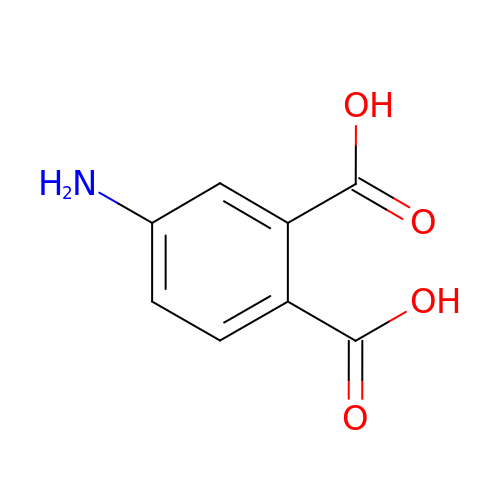4-aminobenzene-1,2-dicarboxylic acid | C8 H7 N O4 | OXSANYRLJHSQEP-UHFFFAOYSA-N>[2x]NAQKRSPTGIVLMNMGGPSKVEETYDFLYQLFADNDLIPISAKYQKTIAKYIAKFRTPKIEKQYREIGGGSPIRKWSEYQATEV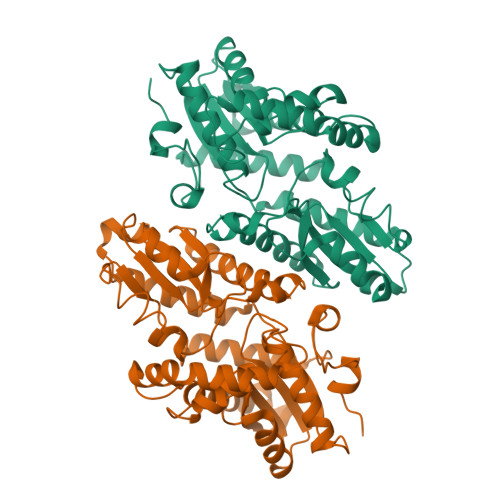CKILDKTCPETAPHKPYVAFRYAKPLTAETYKQMLKDGVKKAVAFSQYPHFSYSTTGSSINELWRQIKALDSERSISWSVIDRWPTNEGLIKAFSENITKKLQEFPQPVRDKVVLLFSAHSLPMDVVNTGDAYPAEVAATVYNIMQKLKFKNPYRLVWQSQVGPKPWLGAQTAEIAEFLGPKVDGLMFIPIAFTSDHIETLHEIDLGVIGESEYKDKFKRCESLNGNQTFIEGMADLVKSHLQSNQLYSNQLPLDFALGKSNDPVKDLSLVFGNHEST ANTHRAMYCIN | C16 H17 N3 O4 | 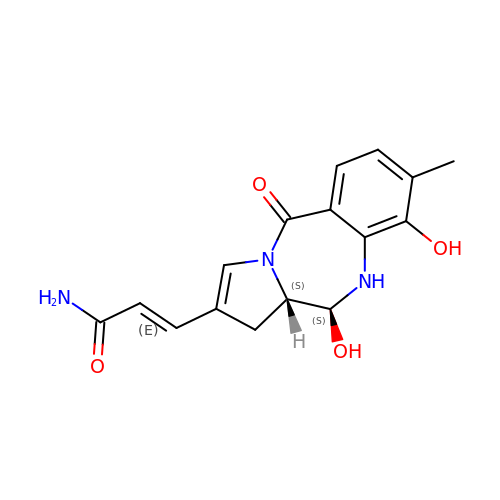VGQOVCHZGQWAOI-HYUHUPJXSA-N TRAF4 belongs to the TRAF family that is composed of seven members in humans. TRAF4 is a modular protein composed of a RING domain, seven TRAF-type zinc-fingers, and a TRAF domain. In this study, we show that TRAF4 uses its TRAF domain as a novel PIP-binding module. To conclude, TRAF4 acts both as a negative regulator of TJs and a cell migration promoter.

The structure was refined to convergence (Rwork = 0.1632, Rfree = 0.1995) and includes residues 283–470 of the TRAF domain. No evidence was seen, however, for the presence of IP4 in the electron density maps. The most striking structural feature of the TRAF domain is the formation of a mushroom-shaped trimer with the coiled-coil domain (TRAF-N) as the stalk and the TRAF-C domain as the cap, which is similar to the described structure of the TRAF domain of TRAF2 and TRAF5. The structural architecture of the TRAF-C domain contains an eight-stranded antiparallel β-sandwich and a three turn helix present in the crossover connection between two β-strands as previously described for TRAF2, TRAF3, and TRAF6 proteins. Altogether, this shows that the recombinant TRAF domain of TRAF4 is well folded and trimerizes in solution similarly to the TRAF domains of TRAF2 and TRAF6. In addition, it can bind up to three PI(3,4,5)P3 molecules, thus suggesting that each TRAF monomer has a binding site for one PIP molecule. We also verified that the overall structure of the K345E mutant was unaffected using gel filtration and dynamic light scattering and showed that this mutant had an organization similar to the WT protein corresponding to a soluble trimer. This mutagenesis study showed that two positive amino acids, lysine 313 and lysine 345, are contributing and essential residues for the binding of TRAF4 to PIPs, respectively. In the model, which was further refined by energy minimization of the fully hydrated protein–ligand complex, the PI(3,4,5)P3-diC4 molecule binds to the TRAF domain at the interface between two protomers. Indeed, the lipid interacts with lysine 313 from one protomer and lysine 345 from the adjacent protomer. Lysine 313 directly interacts with both phosphates at positions 3 and 4 of the PI(3,4,5)P3-diC4, whereas lysine 345 only binds the phosphate at position 5.

>[3x]MALVSRQRQELQELRRELEELSVGSDGVLIWKIGSYGRRLQEAKAKPNLECFSPAFYTHKYGYKLQVSAFLNGNGSGEGTHLSLYIRVLPGAFDNLLEWPFARRVTFSLLDQSDPGLAKPQHVTETFHPDPNWKNFQKPGTWRGSLDESSLGFGYPKFISHQDIRKRNYVRDDAVFIRAAVELPRKILSLEHHHHHH>[2x]GSGDIVSEKKPATEVDPTHFEKRFLKRIRDLGEGHFGKVELCRYDPEGDNTGEQVAVKSLKPESGGNHIADLKKEIEILRNLYHENIVKYKGICTEDGGNGIKLIMEFLPSGSLKEYLPKNKNKINLKQQLKYAVQICKGMDYLGSRQYVHRDLAARNVLVESEHQVKIGDFGLTKAIETDKEYYTVKDDRDSPVFWYAPECLMQSKFYIASDVWSFGVTLHELLTYC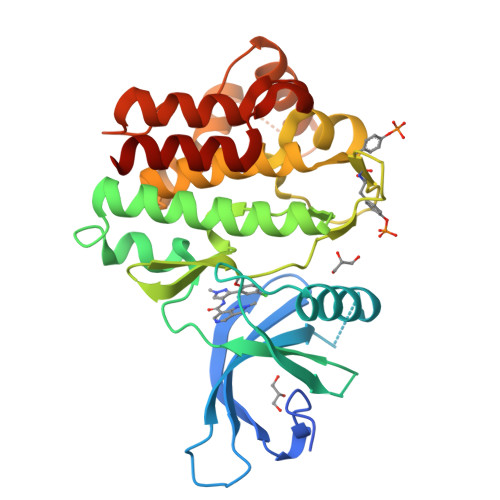DSDSSPMALFLKMIGPTHGQMTVTRLVNTLKEGKRLPCPPNCPDEVYQLMRKCWEFQPSNRTSFQNLIEGFEALLK> MHHHHHHSDACVHHIKRRDIVLKWELGEGAFGKVFLAECHNLLPEQDKMLVAVKALKEASESARQDFQREAELLTMLQHQHIVRFFGVCTEGRPLLMVFEYMRHGDLNRFLRSHGPDAKLLAGGEDVAPGPLGLGQLLAVASQVAAGMVYLAGLHFVHRDLATRNCLVGQGLVVKIGDFGMSRDIYSTDYYRVGGRTML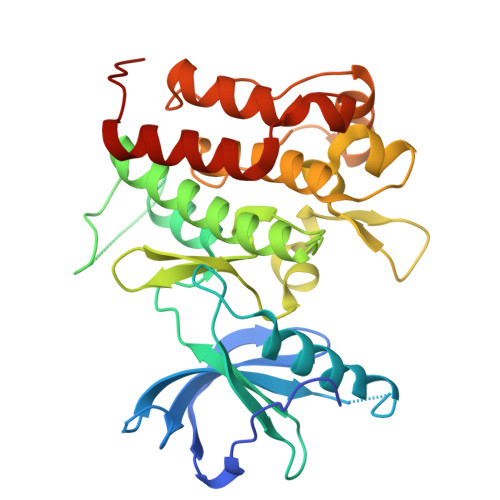PIRWMPPESILYRKFTTESDVWSFGVVLWEIFTYGKQPWYQLSNTEAIDCITQGRELERPRACPPEVYAIMRGCWQREPQQRHSIKDVHARLQALAQAPPVYLDVLG2-(methylamino)-1H-benzimidazole-5-carboxamide 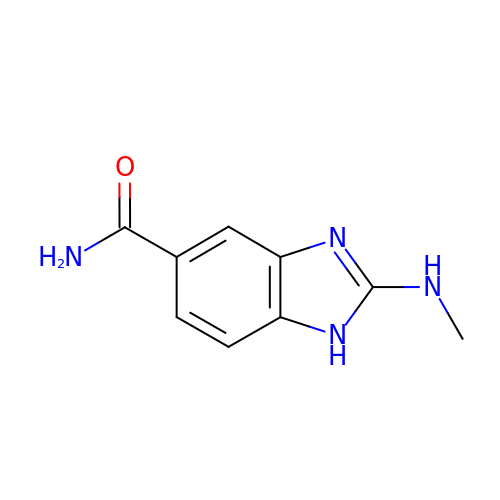| C9 H10 N4 O | LOKXPWIZESGCLZ-UHFFFAOYSA-N>[4x]ARSTNTFNYATYHTL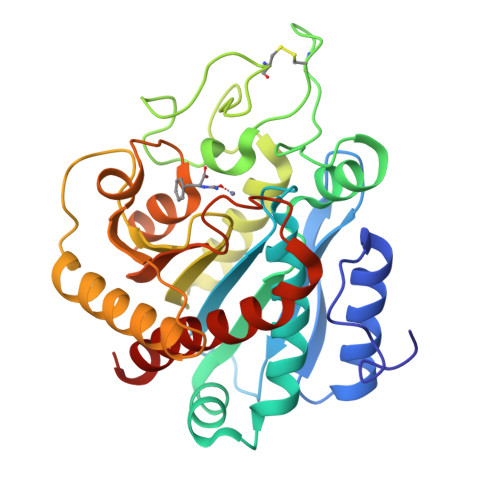DEIYDFMDLLVAQHPELVSKLQIGRSYEGRPIYVLKFSTGGSNRPAIWIDLGIHSREWITQATGVWFAKKFTENYGQNPSFTAILDSMDIFLEIVTNPNGFAFTHSENRLWRKTRSVTSSSLCVGVDANRNWDAGFGKAGASSSPCSETYHGKYANSEVEVKSIVDFVKNHGNFKAFLSIHSYSQLLLYPYGYTTQSIPDKTELNQVAKSAVAALKSLYGTSYKYGSIITTIYQASGGSIDWSYNQGIKYSFTFELRDTGRYGFLLPASQIIPTAQETWLGVLTIMEHTVNN> LKLSAENESTPIQQLLEHFLRQLQRKDPHGFFAFPVTDAIAPGYSMIIKHPMDFGTMKDKIVANEYKS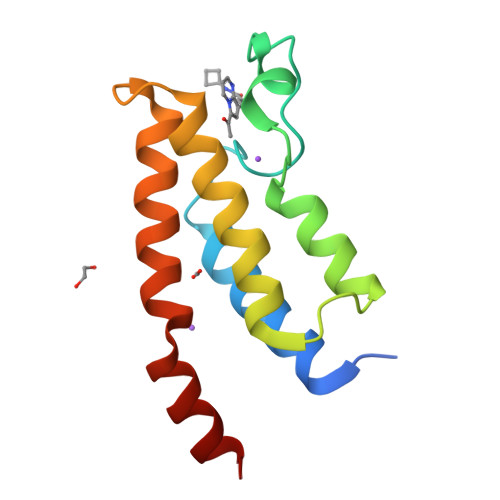VTEFKADFKLMCDNAMTYNRPDTVYYKLAKKILHAGFKMMSKERLLALKRSMS(2S,3R,4S,5S)-2-methyl-5-(4-methylphenyl)pyrrolidine-3,4-diol 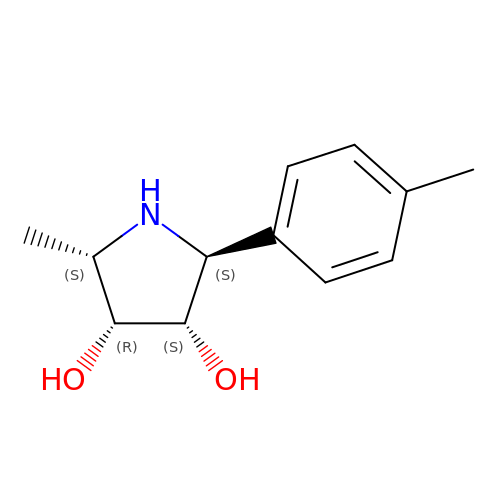| C12 H17 N O2 | VSLJKQDKGOXAQN-IXLVHKGHSA-N> MALHYFLQYDVQILCIALMFSIFRVCIS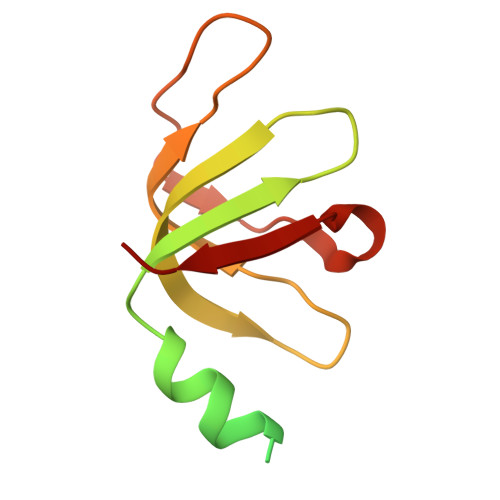TAIDFTSPKLDEFSLIMEMGEILLTSWLNRSVHIEIFDERKFIGKFLCTDREGAAILSNTTEYNKGFSRALGLVVIPGKHIKSFSVRA[(2~{R},3~{R},4~{R},5~{S},6~{R})-3-acetamido-6-(hydroxymethyl)-4,5-bis(oxidanyl)oxan-2-yl] [oxidanyl-[(2~{Z},6~{Z},10~{Z})-3,7,11,15-tetramethylhexadeca-2,6,10,14-tetraenoxy]phosphoryl] hydrogen phosphate | C28 H49 N O12 P2 | 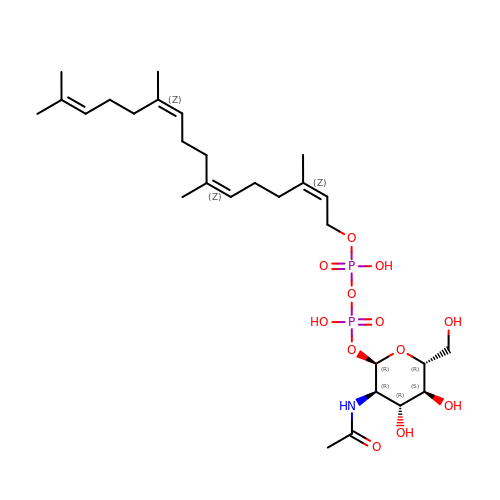MCKZOQNLWLVDRX-ADLZVGHSSA-N> MGSDKIHHHHHHMYETFMKRAIELAKKGLGRVNPNPPVGAVVVKDGRIIAEGFHPYFGGPHAERMAIESARKKGEDLRGATLIVTLE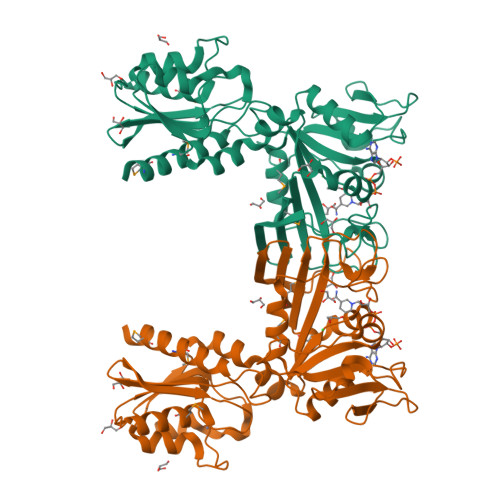PCDHHGKTPPCTDLIIESGIKTVVIGTRDPNPVSGNGVEKFRNHGIEVIEGVLEEEVKKLCEFFITYVTKKRPFVALKYASTLDGKIADHRGDSKWITDKLRFKVHEMRNIYSAVLVGAGTVLKDNPQLTCRLKEGRNPVRVILDRKGVLSGKVFRVFEENARVIVFTESEEAEYPPHVEKALSDCSVESILRNLYERDIDSVLVEGGSKVFSEFLDHADVVFGFYSTKIFGKGLDVFSGYLSDVSVPPKFKVVNVEFSDSEFLVEMRPCSRE> GPLGSKDTRPQTDDVLNTKGNTFEDFYLKRELLMGIFEAGFEKPSPIQEEAIPVAITGRDILARAKNGTGKTAAFVIPTLEKVKPKLNKIQALIMVPTRELALQTSQVVRTLGKHCGISCMVTTGGTNLRDDILRLNETVHILVGTPGRVLDLASRKVADLSDCSLFIMDEADKMLSRDFKTIIEQILSFLPPTHQSLLFSATFPLTVKEFMVKHLHKPYEINLMEELTLKGITQYYAFVEERQKLHCLNTLFSKLQINQAIIFCNSTNRVELLAKKITDLGYSCYYSHARMKQQERNKVFHEFRQGKVRTLVCSDLLTRGIDIQAVNVVINFDFPKTAETYLHRIGRSGRFGHLGLAINLINWNDRFNLYKIEQELGTEIAAIPATIDKSLYVAEN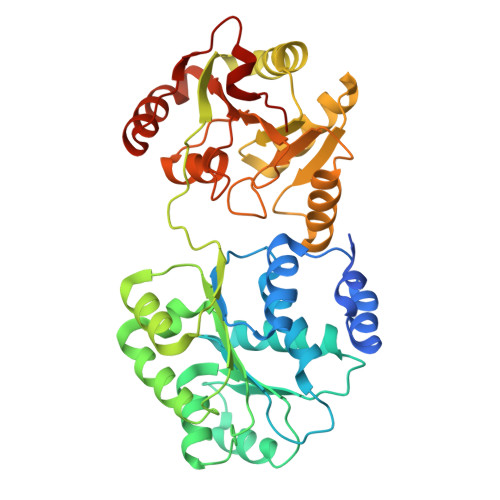DET> GAMLYLIFYDITDDNLRNRVAEFLKKKGLDRIQYSVFMGDLNSSRLKDVEAGLKIIGNRKKLQEDERFFILIVPITENQFR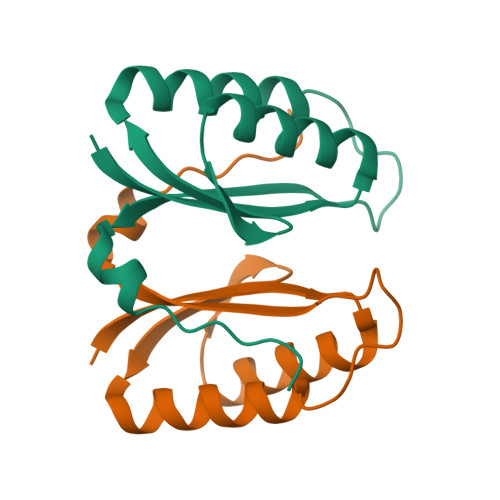ERIVIGYSGSEREEKSNVVW> MDNVDFAESVRTRWARRLIREKVAKELNILTERLGEVPGIPPPREGRFLGGGYSHDNLPSDPLYSSIKPALLKEAPRAEEELPPRKVCIVGAGVSGLYIAMILDDLKIPNLTYDIFESSSRTGGRLYTHHFTDAKHDYYDIGAMRYPDIPSMKRTFNLFKRTGMPLIKYYLDGENTPQLYNNHFFAKGVVDPYMVSVANGGTVPDDVVDSVGEKLQQAFGYYKEKLAEDFDKGFDELMLVDDMTTREYLKRGGPKGEAPKYDFFAIQWMETQNTGTNLFDQAFSESVIDSFDFDNPTKPEWYCIEGGTSLLVDAMKETLVHKVQNNKRVEAISIDLDAPDDGNMSVKIGGKDYSGYSTVFNTTALGCLDRMDLRGLNLHPTQADAIRCLHYDNSTKVALKFSYPWWIKDCGITCGGAASTDLPLRTCVYPSYNLGDTGEAVLLASYTWSQDATRIGSLVKDAPPQPPKEDELVELILQNLARLHAEHMTYEKIKEAYTGVYHAYCWANDPNVGGAFALFGPGQFSNLYPYLMRPAAGGKFHIVGEASSVHHAWIIGSLESAYTAVYQFLYKYKMWDYLRLLLERWQYGLQELETGKHGTAHLQFILGSLPKEYQVKI

l-Lysine oxidase (LysOX) is a member of the LAAO family protein and has strict substrate specificity for l-lysine. LysOX from Trichoderma viride is synthesized as a precursor (prLysOX) and the N-terminal 77 residues are cleaved to produce the mature protein composed of 540 amino acid residues. The mature enzyme consists of three domains; the FAD-binding domain, the helical domain, and the substrate-binding domain. The active site is present at the bottom of the funnel formed between the substrate-binding domain and the helical domain.

The crystal structure of prLysOX was determined at 1.97 Å resolution. A single prLysOX molecule is in an asymmetric unit and forms a dimer with the neighboring molecule related by crystallographic two-fold symmetry. prLysOX consists of 617 amino acid residues, and the final model contains N3–R44, G51–A70, and E79–K611. The propeptide (M1–R77) of LysOX folds into a sub-domain on the FAD-binding domain with the C-terminal region (Q590–K611), which is disordered in the mature LysOX structure. The propeptide region consists of an 8-turn amphiphilic α-helix (F6–L34, αN), a proline/glycine-rich region that forms a repeat of turn structures (G35–P62), and a loop with a short helical segment (L63–R72). Unlike the precursor of PAO, the propeptide is far from the entrance of the funnel leading to the active site. The propeptide induces a structural change in the helical domain, but no significant change is found in the other two domains. αN is inserted between the helical domain and the FAD-binding domain. The N-terminal region of αN pushes up α5 and α6 resulted in straightening the kink between α4 and α5 and induces a movement of α9 to form a tight hydrophobic interaction. The movement of α9 changes the shape of the active site. D289 and F293 in α9 move away from the active site. T276 in the loop connecting α8 and α9 moves to space where the water mediating the interaction between the ε-amino group of l-lysine and D392 existed.>[4x]MSQHNEKNPHQHQSPLHDSSEAKPGMDSLAPEDGSHRPAAEPTPPGAQPTAPGSLKAPDTRNEKLNSLEDVRKGSENYALTTNQGVRIADDQNSLRAGSRGPTLLEDFILREKITHFDHERIPERIVHARGSAAHGYFQPYKSLSDITKADFLSDPNKITPVFVRFSTVQGGAGSADTVRDIRGFATKFYTEEGIFDLVGNNTPIFFIQDAHKFPDFVHAVKPEPHWAIPQGQSAHDTFWDYVSLQPETLHN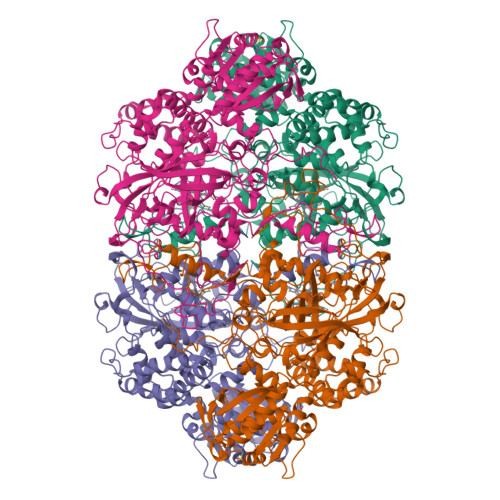VMWAMSDRGIPRSYRTMEGFGIHTFRLINAEGKATFVRFHWKPLAGKASLVWDEAQKLTGRDPDFHRRELWEAIEAGDFPEYELGFQLIPEEDEFKFDFDLLDPTKLIPEELVPVQRVGKMVLNRNPDNFFAENEQAAFHPGHIVPGLDFTNDPLLQGRLKSYTDTQISRLGGPNFHEIPINRPTCPYHNFQRDGMHRMGIDTNPANYEPNSINDNWPRETPPGPKRGGFESYQERVEGNKVRERSPSFGEYYSHPRLFWLSQTPFEQRHIVDGFSFELSKVVRPYIRERVVDQLAHIDLTLAQAVAKNLGIELTDDQLNITPPPDVNGLKKDPSLSLYAIPDGDVKGRVVAILLNDEVRSADLLAILKALKAKGVHAKLLYSRMGEVTADDGTVLPIAATFAGAPSLTVDAVIVPCGNIADIADNGDANYYLMEAYKHLKPIALAGDARKFKATIKIADQGEEGIVEADSADGSFMDELLTLMAAHRVWSRIPKIDKIPA Acid sphingomyelinase (ASMase, ASM, SMPD1) is an enzyme found in lysosomes and in the extracellular space where it catalyses the conversion of sphingomyelin, a major component of membranes, into ceramide and phosphocholine. ASMase consists of an N-terminal saposin domain and a C-terminal catalytic domain. To gain insight into the molecular mechanism of ASMase function and the interplay between its domains, we determined crystal structures of the full-length protein from mouse that reveal a conformational flexibility of the saposin domain. In one conformation, the saposin domain adopts a globular closed form independent of the catalytic domain, while in the other conformation, it assumes an open V-shaped fold that establishes an extended interface with the catalytic domain.

As observed with other saposins, ASMasesap adopts either a closed or open conformation depending on environmental conditions. In the closed form, ASMasesap is compact, globular and interacts mainly with the CTD, although this interaction appears to be a consequence of the crystal lattice since the two molecules in the asymmetric unit occupy slightly different positions, with the linker between the domains disordered in one molecule. In the absence of membranes, closed ASMasesap decoupled from ASMasecat would predominate and render the enzyme inactive. To further these efforts, we determined the structure of ASMase bound to a known high-affinity inhibitor, 1-aminodecylidene bis-phosphonic acid (AbPA; half-maximal inhibitory concentration 20 nM)24. One phosphate group of AbPA completes the coordination shell for the zinc ions whereas its nine-carbon lipid tail sits in a relatively featureless shallow groove. This structure and the position of the leaving group-protonating His280 allowed us to propose a model for how sphingomyelin might bind to the active site. The fatty-acid chains of sphingomyelin sit along a hydrophobic track that extends from the edge of the active site to the saposin domain and surprisingly, do not correspond to the position of the AbPA lipid tail, which instead coincides with the position of the choline head group. These results will help direct the rational design of new ASMase inhibitors that better exploit the shape of the active site.

>[2x]DRHHHHHHKLNLTCPACKVLFTALNHGLKKEPNVARVGSVAIKICKMLNIAPLDVCQSAVHLFEDDVVEVWTRSVLSPSEACGLLLGSSCGHWDIFSTWNISLPSVPKPPPKPPSPPAPGAPVSRVLFLTDLHWDHEYLEGTDPYCADPLCCRRGSGWPPNSQKGAGFWGEYSKCDLPLRTLESLLKGLGPAGPFEMVYWTGDIPAHDVWQQSRQDQLRALTTITDLVRKFLGPVPVYPAVGNHESTPVNGFPPPFIKGNQSSQWLYEAMAKAWEPWLPADALHTLRIGGFYALTPRPGLRLISLNMNFCSRENFWLLINSTDPAGQLQWLVEELQAAENRGDKVHIIGHIPPGHCLKSWSWNYYKIIARYENTLAGQFFGHTHVDEFEIFYDEETLSRPLAVAFLAPSATTFINLNPGYRVYQIDGNYPGSSHVVLDHETYILNLTQANAAGGTPSWKRLYRARETYGLPDAMPASWHNLVYRMRDDEQLFQTFWFLYHKGHPPSEPCGTPCRLATLCAQLSARADSPALCRHLMPN>[2x]QDADKLPHTKVTLVAPPQVHPHEQATKSGPKVVEFTMTIEEKKMVIDDKGTT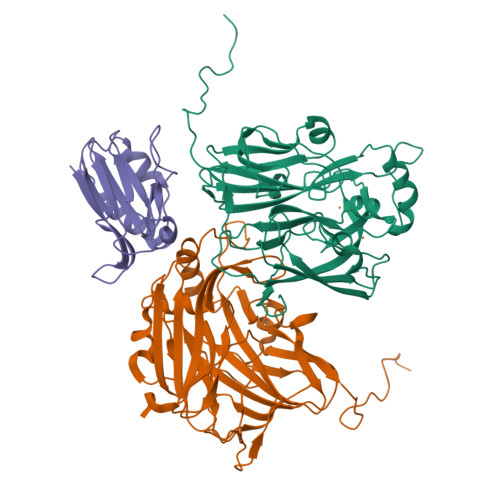LQAMTFNGSMPGPTLVVHEGDYVQLTLVNPATNAMPHNVDFHGATGALGGAKLTNVNPGEQATLRFKADRSGTFVYHCAPEGMVPWHVVSGMSGTLMVLPRDGLKDPQGKPLHYDRAYTIGEFDLYIPKGPDGKYKDYATLAESYGDTVQVMRTLTPSHIVFNGKVGALTGANALTAKVGETVLLIHSQANRDTRPHLIGGHGDWVWETGKFANPPQRDLETWFIRGGSAGAALYTFKQPGVYAYLNHNLIEAFELGAAGHIKVEGKWNDDLMKQIKAPAPIPR;> AEHIVEMRNKDDAGNTMVFQPGFVKVEAGDTVKFVPTDKSHNAESVREVWPEGVAPVKGGFSKEVVFNAEKEGLYVLKCAPHYGMGMVVLVQVGKPVNLDQIKEYKATGLAKKRLDGEIAKVVQ> QRTKIVVKVHMPCGKSRAKALALAASVNGVDSVEITGEDKDRLVVVGRGIDPVRLVALLREKCGLAELLMVELVK;> I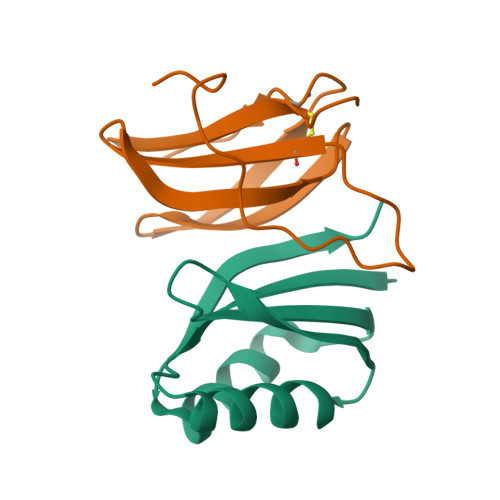DLSRERDPNFFDHPGIPVPECFWFMFKNNVRQDAGTCYSSWKMDMKVGPNWVHIKSDDNCNLSGDFPPGWIVLGKKRPGF> MGSAMSLGCSKRKATNQDVDSESRKRRKICSTNDAENCRFIQDESSWKHPWSLCANSVVNDTKDTKSSALSLPSPPTSVSRIWKHQVFPSFHGADVRKTILSHILESFRRKGIDPFIDNNIERSKSIGHELKEAIKGSKIAIVLLSKNYASSSWCLDELAEIMKCRELLGQIVMTIFYEVDPTDIKKQTGEFGKAFTKTCKGKTKEYVERWR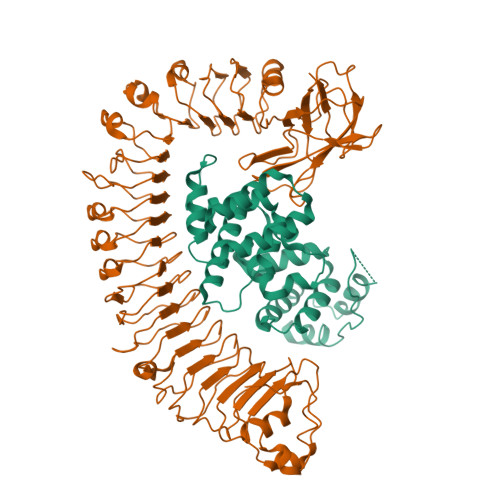KALEDVATIAGYHSHKWRNEADMIEKIATDVSNMLNSFKPSRDFNGLVGMRAHMDMLEQLLRLVLDEVRMIGIWGPPGIGKTTIARFLFNQVSDRFQLSAIMVNIKGCYPRPCFDEYSAQLQLQNQMLSQMINHKDIMISHLGVAQERLRDKKVFLVLDEVDQLGQLDALAKETRWFGPGSRIIITTEDLGVLKAHGINHVYKVGYPSNDEAFQIFCMNAFGQKQPHEGFDEIAREVMALAGELPLGLKVLGSALRGKSKPEWERTLPRLKTSLDGKIGSIIQFSYDALCDEDKYLFLYIACLFNKESTTKVEGLLGKFLDVRQGLHILAQKSLISIEDGNIYMHTLLEQFGRETSRKQFIHHGYTKHQLLVGERDICEVLNDDTIDSRRFIGINLDLYKNVEELNISEKALERIHDFQFVRINGKNHALHERLQGLIYQSPQIRSLHWKCYQNICLPSTFNSEFLVELDMSFSKLQKLWEGTKQLRNLKWMDLSYSSYLKELPNLSTATNLEELKLRNCSSLVELPSSIEKLTSLQILDLHRCSSLVELPSFGNATKLEILNLENCSSLVKLPPSINANNLQELSLTNCSRVVELPAIENATNLWKLNLLNCSSLIELPLSIGTATNLKHLDFRGCSSLVKLPSSIGDMTNLEVFYLSNCSNLVELPSSIGNLRKLTLLLMRGCSKLETLPTNINLKSLHTLNLIDCSRLKSFPEISTHIKYLRLIGTAIKEVPLSIMSWSPLAHFQISYFESLKEFPHALDIITELQLSKDIQEVPPWVKRMSRLRALRLNNCNNLVSLPQLPDSLAYLYADNCKSLERLDCCFNNPEIRLYFPKCFKLNQEARDLIMHTSTRNFAMLPGTQVPACFNHRATSGDSLKIKLKESPLPTTLTFKACIMLVNEEMSYDLKSMSVDIVIRDEQNDLKVQCTPSYHQCTEIYVLTEHIYTFELEVEEVTSTELVFEFTSVNESICKIGECGILQRETRSLRRSSSPDLSPESSRVSSCDHC;> MRVCYFVLVPSVALAVIATESSETSGTIVHVFPLRDVADHRNDALINRALRAQTALDDDEERWPFGPSAVEALIETIDRHGRVSLNDEAKMKKVVRTWKKLIERDDLIGEIGKHYFEAPGPLHDTYDEALATRLVTTYSDRGVARAILHTRPSDPLSKKAGQAHRLEEAVASLWKGRGYTSDNVVSSIATGHDVDFFAPTAFTFLVKCVESEDDANNAIFEYFGSNPSRYFSAVLHAMEKPDADSRVLESSKKWMFQCYAQKQFPTPVFERTLAAYQSEDYAIRGARNHYEKLSLSQIEELVEEYSRIYSV>[2x]MSQPRTPEQALDTPGDCPPGRRDEDAGEGIQCSQRMLSFSDALLSIIATVMILPVTHTEISPEQQFDRSVQRLLATRIAVYLMTFLIVTVAWAAHTRLFQVVGKTDDTLALLNLACMMTITFLPYTFSLMVTFPDVPLGIFLFCVCVIAIGVVQALIVGYAFHFPHLLSPQIQRSAHRALYRRHVLGIVLQGPALCFAAAIFSLFFVPLSYLLMVTVILLPYVSKVTGWCRDRLLGHREPSAHPVEVFSFDLHEPLSKERVEAFSDGVYAIVATLLILDICEDNVPDPKDVKERFSGSLVAALSATGPRFLAYFGSFATVGLLWFAHHSLFLHVRKATRAMGLLNTLSLAFVGGLPLAYQQTSAFARQPRDELERVRVSCTIIFLASIFQLAMWTTALLHQAETLQPSVWFGGREHVLMFAKLALYPCASLLAFASTCLLSRFSVGIFHLMQIAVPCAFLLLRLLVGLALATLRVLRGLARPEHPPPAPTGQDDPQSQLLPAPC

Transmembrane protein 175 (TMEM175) is a potassium (K+)-selective cation channel that is evolutionarily distinct from all other known ion channels. In mammals, TMEM175 is expressed in lysosomes, where it is critical for maintaining lysosomal homeostasis. To begin to understand the mechanisms that underlie TMEM175 function in lysosomes, we determined the structure of hTMEM175 by cryo-EM and identified two conformational states. hTMEM175 protomers consist of two homologous repeats of six TM helices, which assemble into a dimer to form the channel. A 2-fold symmetric ion conduction pathway runs along the center of the dimer, lined by two copies of TM1 and TM7, the first helices of each repeat.

The resolution of the putative open state improved from 2.64 to 2.45 Å and the closed state improved from 3.03 to 2.61 Å. In the closed state, the isoleucine constriction formed by Ile46 and Ile271 is too narrow to allow ion permeation. The side chains of Ile271 point toward the channel axis, narrowing the pore to a minimum radius of 0.2 Å. For the closed state, we can now model three ion-binding sites and 25 water molecules into non-protein densities. In the cytosolic region of the pore, where the channel undergoes minimal conformational changes during gating, the K1 and K2 ion-binding sites and water molecules occupy almost identical positions to those resolved in the open state. In contrast, there is little correspondence between the ion and water configurations at the isoleucine constriction or on the luminal side of the pore due to the conformational changes that occur to the channel during channel gating. The inward movement of Ile271 displaces the ion-binding sites on either side of the isoleucine constriction. Movements of Thr49 and Thr274, which both coordinate water molecules in the open state, result in a movement of the luminal K5 ion-binding site toward the luminal entrance of the pore. Thus, the higher-resolution structures reveal how changes in the protein structure alter the ion conduction pathway to prevent ion permeation in the closed state.Like the scCST, the hCST (Ctc1, hStn1 and hTen1) complex is predicted to contain multiple OB-folds and it binds telomeric overhangs with high affinity and some specificity. Overall, hCST plays a role in telomere replication, and may also have a more general role under conditions of replicative stress. To further elucidate the role of hCST at the telomeres, we solved the structures of hTen1 in complex with the N-terminal domain of hStn1 (hStn1N), and the C-terminal domain of hStn1 (hStn1C) alone. These structures reveal that hStn1-Ten1 is a RPA-like complex and a structural homologue of Schizosaccharomyces pombe Stn1Ten1 (spStn1Ten1) and Candida tropicalis Stn1Ten1 (ctStn1Ten1).

A search in the PDB database using the Dali server shows that the structure of the hStn1N-Ten1 complex is strikingly similar to the S. pombe and C. tropicalis Stn1-Ten1 telomeric complexes with an RMSD of 2.1 Å and 2.9 Å respectively, indicating significant structural conservation of these telomeric complexes between humans and spStn1Ten1 and ctStn1Ten1. We observed that the hStn1-Ten1 complex has striking structural similarities to both spStn1-Ten1 and ctStn1-Ten1. This close structural relationship indicates that they likely carry out a conserved function at telomeres. Many of the conserved residues making contacts between hStn1N and hTen1 are located on the C-terminal helices and the β-barrels of these proteins. To determine the role of hStn1-Ten1 complex assembly in telomere function we designed single and double mutants of conserved residues required for hStn1-Ten1 heterodimerization. Functional assays of hStn1 mutants defective for hTen1 binding show telomere signal-free ends, longer and fragile telomeres, phenotypes associated with telomere length deregulation and a dysfunctional scCST complex. DNA binding assays reveal that hStn1 shows a robust ssDNA binding activity while hTen1 binds ssDNA at a non-appreciable level (≥15 µM). Interestingly, the hStn1-Ten1 complex exhibited non-specific ssDNA binding activity but with an affinity lower than that observed for hStn1 alone. The OB fold of RPA32 (hStn1 homologue) is a DNA binding domain that is involved in the 30 nucleotide binding mode of RPA, and helps the complex to achieve its 0.1 nM binding affinity for ssDNA while RPA14 (hTen1 homologue) is not involved in high-affinity DNA binding. It's possible then that hTen1 carries out primarily a structural role in hCST assembly thus enhancing Ctc1 and hStn1 DNA binding via promoting the proper assembly of the trimeric CST complex.

>LDPVFLAFAKLYIRDILDMKESRQVPGVFLYNGHPIKQVDVLGTVIGVRERDAFYSYGVDDSTGVINCICWKKLNTESVSAAPSAARELSLTSQLKKLQETIEQKTKIEIGDTIRVRGSIRTYREEREIHATTYYKVDDPVWNIQIARMLELPTIYRKVYDQPFHS[2x];>[2x]MLPKPGTYYLPWEVSAGQVPDGSTLRTFGRLCLYDMIQSRVTLMAQHGSDQHQVLVCTKLVEPFHAQVGSLYIVLGELQHQQDRGSVVKARVLTCVEGMNLPLLEQAIREQRLYKQERGGSQ In eukaryotes, primers are generated by the heterotetrameric DNA polymerase α-primase (pol-prim) complex, which possesses two enzymatic activities in two distinct active sites. Primase, a DNA-dependent RNA polymerase, generates the initial hybrid RNA-DNA primed substrate, which is then handed off to DNA polymerase α (pol α) to extend the initial primer by approximately twenty DNA nts. Human DNA primase is composed of catalytic (p48) and regulatory (p58) subunits. The regulatory subunit has a C-terminal domain (p58C) that is unique to higher eukaryotes and contains a [4Fe4S] cluster.

To test if the differences between the p58C266-456 and p58C272-464 structures were a by-product of the differences in sequence, we produced, purified, and crystallized a p58C construct containing residues 266–464 in the conditions used to crystallize p58C272-464. With these residues omitted, density for residues in extended conformation that together formed a beta-type interaction were clearly evident in the p58C266-464 2Fo-Fc map. As previously observed for p58C272-464 under these conditions, crystallized as a dimer, with a disulfide cross-link between the two Cys449 residues and several stabilizing interactions between symmetry-related molecules. In p58C266-464, residues 330–340 and 353–360 in chain A and 330–345 and 353–359 in chain B are missing due to disorder. A best-fit superposition of the two structures reveals they are very similar, with a backbone RMSD of only 0.23 Å. This finding shows that the differences in residues Leu318-His351 evident from comparing the previous p58C structures are not intrinsic to the differences in the N-termini of the constructs but rather to differences in the crystallization conditions. Analysis of the p58C266-464 and p58C272-464 crystal structures reveals that substantial crystal lattice packing interactions stabilize this region in both structures. Specifically, Leu318-Gln329 are seen to interact extensively with the same region in the adjacent molecule in the lattice. In addition, on both sides of this extended interaction, Phe326 completes a hydrophobic pocket in the adjacent molecule, providing an additional anchor between the two molecules.

>GNVGKISLDQIDLLSTKSFPPCMRQLHKALRENHHLRHGGRMQYGLFLKGIGLTLEQALQFWKQEFIKGKMDPDKFDKGYSYNIRHSFGKEGKRTDYTPFSCLKIILSNPPSQGDYHGCPFRHSDPELLKQKLQSYKISPGGISQILDLVKGTHYQVACQKYFEMIHNVDDCGFSLNHPNQFFCESQRILNG[2x]>MASWSHPQFEKGAMTARKVDYTDGATRCIGEFHWDEGKSGPRPGVVVFPEAFGLNDHAKERARRLADLGFAALAADMHGDAQVFDAASLSSTIQGYYGDRAHWRRRAQAALDALTAQPEVDGSKVAAIGFCFGGATCLEL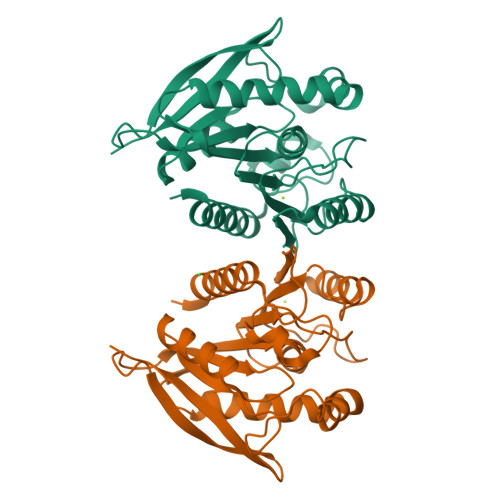ARTGAPLTAIVTFHGGLLPEMAGDAGRIQSSVLVCHGADDPLVQDETMKAVMDEFRRDKVDWQVLYLGNAVHSFTDPLAGSHGIPGLAYDATAEARSWTAMCNLFSELFG[2x]> XDSTTEGTPADGF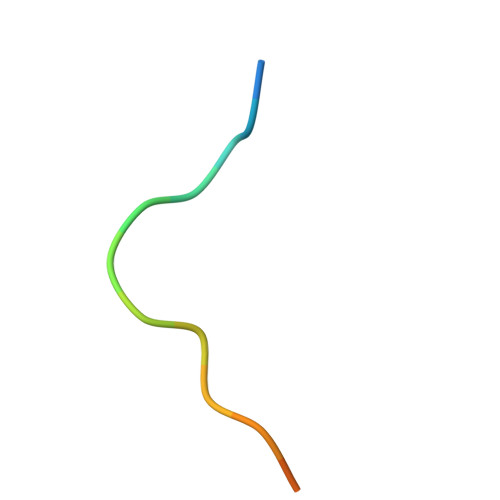TVL> MHHHHHHSSGRENLYFQGIAINPGMYVRKKEGKIGESYFKVRKLGSGAYGEVLLCKEKNGHSEKAIKVIKKSQFDKGRYSDDNKNIEKFHEEIYNEISLLKSLDHPNIIKLFDVFEDKKYFYLVTEFYEGGELFEQIINRHKFDECDAANIMKQILSGICYLHKHNIVHRDIKPENILLENKNSLLNIKIVDFGLSSFFSKDYKLRDRLGTAYYIAPEVLKKKYNEKCDVWSCGVIMYILLCGYPPFGGQNDQDIIKKVEKGKYYFDFNDWKNISDEAKELIKLMLTYDYNKRCTAEEALNSRWIKKYANNINKSDQKTLCGALSNMRKFEGSQKLAQAAILFIGSKLTTLEERKELTDIFKKLDKNGDGQLDKKELIEGYNVLRNFKNELGELKNVEEEVDNILKEVDFDKNGYIEY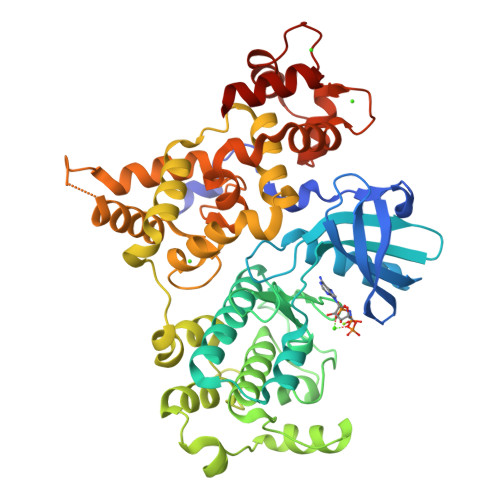SEFISVCMDKQILFSEERLRRAFNLFDTDKSGKITKEELANLFGLTSISEKTWNDVLGEADQNKDNMIDFDEFVSMMHKICDHKTF> ARPAAEDPPRDKFAGDRAPTRP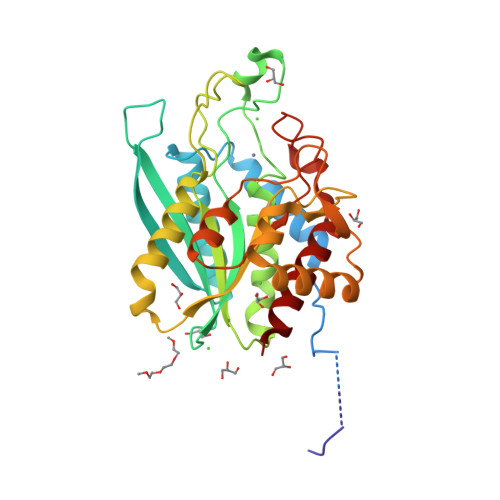DGDGGLKRDKFGEDRVPTKPDFKTFPLDPDRAVKYVQQLCDIGPRISGTPGMVKQQEVLTKHFEGLGAKVVRQEFKVRQRSQRGAVDMTNLIASWFPDRKARLIVCSHYDTRPAAHQETDTQNWRKPFASANDGTAGAALMMELAHHMKGVPSNVGVDFVLFDGEEYILDPGVPGLQEGDKYFFGSEHFANGYTKAKAGLPYRYTGAVLLDLFAHDGARLAMEGYSLRGAPNLVAELWRVAGWVGAKSFVNERGFDRATDVLDDHIALNEAGIPAVDVIDFDYKHWHLLSDTPDKISGKQMVDVGNVLLGWIQIQK>[2x]GSDYIIKEKTVLLQKKDSEGFGFVLRGAKAQTPIEEFTPTPAFPALQY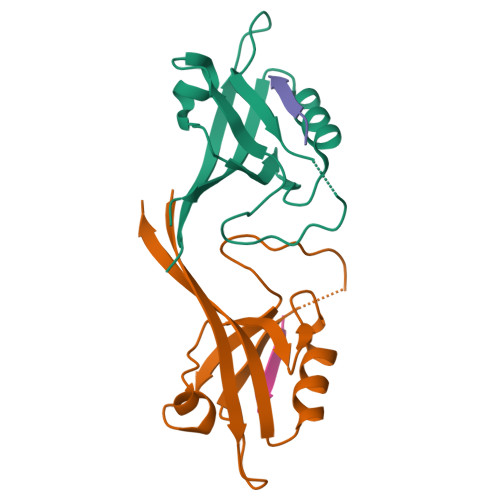LESVDEGGVAWRAGLRMGDFLIEVNGQNVVKVGHRQVVNMIRQGGNTLMVKVVMVTRHPDM;>[2x]EAQTRL> GNSKSGALSKEILEELQLNTKFTE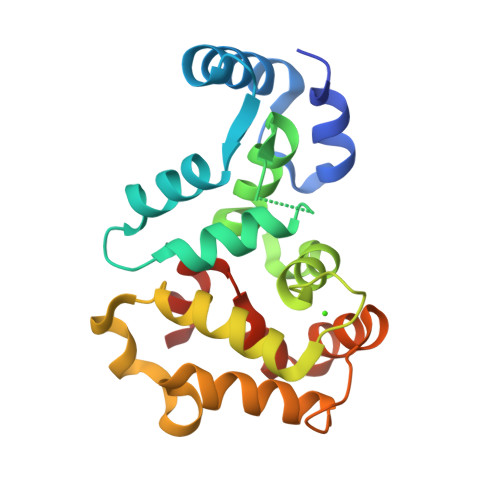EELSSWYQSFLKECPSGRITRQEFQTIYSKFFPEADPKAYAQHVFRSFDANSDGTLDFKQYVIALHMTSAGKTNQKLEWAFSLYDVDGNGTISKNEVLEIVTAIFKMISPEDTKHLPEDENTPEKRAEKIWGFFGKKDDDKLTEKEFIEGTLANKEILRLIQFEPQKVKEKLKEKKL>MFEIKKICCIGAGYVGGPTCSVIAHMCPEIRVTVVDVNESRINAWNSPTLPIYEPGLKEVVESCRGKNLFFSTNIDDAIKEADLVFISVNTPTKTYGMGKGRAADLKYIEACARRIVQNSNGYKIVTEKSTVPVRAAESIRRIFDANTKPNLNLQVLSNPEFLAEGTAIKDLKNPDRVLIGGDETPEGQRAVQALCAVYEHWVPREKILTTNTWSSELSKLAANAFLAQRISSINSISALCEATGADVEEVATAIGMDQRIGNKFLKASVGFGGSCFQ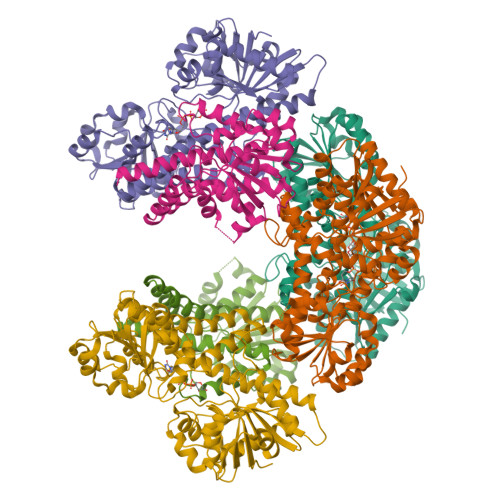KDVLNLVYLCEALNLPEVARYWQQVIDMNDYQRRRFASRIIDSLFNTVTDKKIAILGFAFKKDTGDTRESSSIYISKYLMDEGAHLHIYDPKVPREQIVVDLSHPGVSEDDQVSRLVTISKDPYEACDGAHAVVICTEWDMFKELDYERIHKKMLKPAFIFDGRRVLDGLHNELQTIGFQIETIGKKVSSKRIPYAPSGEIPKFSLQDPPNKKPKV[6x]>[4x]MSLNADFATEIEGKIVQA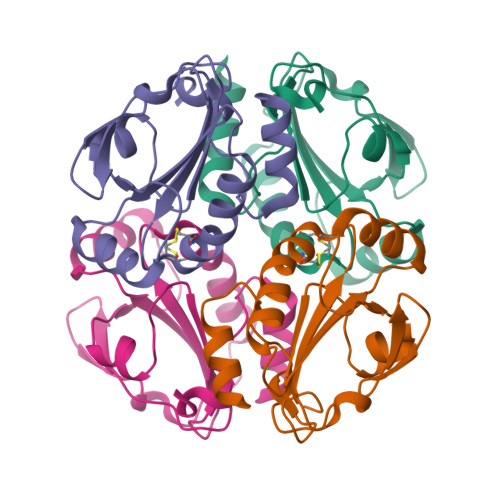SKLLPGQPAIDFEMLDVEGNVKHLADFKGKVIYIDLWATWCGPCIQESPAFEALGKKYVGKDIVFLPVSTDTTTKPWLRYLDGHKKELTQYHSNDVALKESWAIMYIPRFILIDKDFNIVNAYAPRPSSEEIGTLIDSVLNKEGHHHHHH>MGHHHHHHHHHHSSGHIEGRHMYTVMLDLKGRSVLVVGGGTIATRRIKGFLQEGAAITVVAPTVSAEINEWEAKGQLRVKRKKVGEEDLLNVFFIVVATNDQAVNKFVKQHIKNDQLVNMASSFSDGNIQIPAQFSRG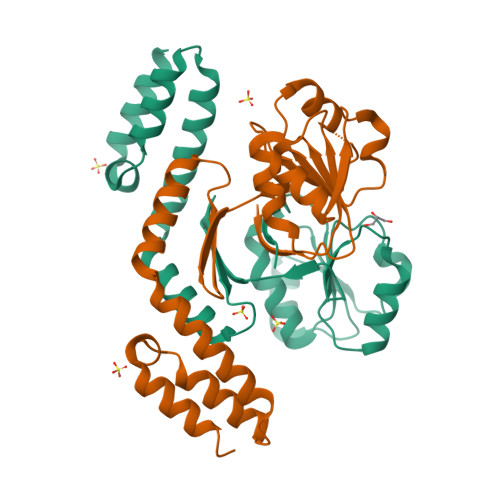RLSLAISTDGASPLLTKRIKEDLSSNYDESYTQYTQFLYECRVLIHRLNVSKSRKHELLTEIIDDQYRLSLVKQREFLQQIEKYK[2x]>[2x]MHHHHHHDSKHQCVKLNDGHFMPVLGFGTYAPPEVPRSKALEVTKLAIEAGFRHIDSAHLYNNEEQVGLAIRSKIADGSVKREDIFYTSKLWSTFHRPELVRPALENSLKKAQLDYVDLYLIHSPMSLKPGEELSPTDENGKVIFDIVDLCTTWEAMEKCKDAGLAKSIGVSNFNRRQLEMILNKPGLKYKPVCNQVECHPYFNRSK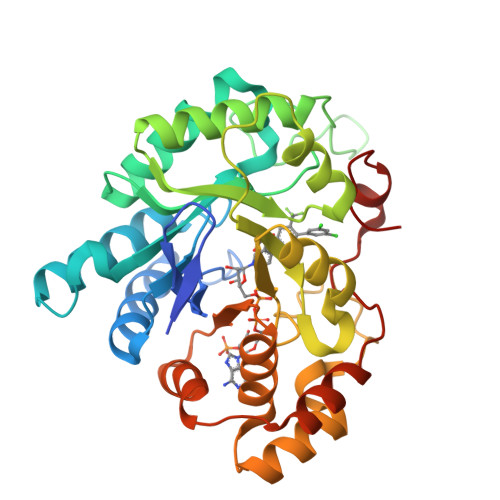LLDFCKSKDIVLVAYSALGSQRDKRWVDPNSPVLLEDPVLCALAKKHKRTPALIALRYQLQRGVVVLAKSYNEQRIRQNVQVFEFQLTAEDMKAIDGLDRNLHYFNSDSFASHPNYPYSDEY5-(1H-pyrrolo[2,3-b]pyridin-3-ylmethyl)-N-[4-(trifluoromethyl)benzyl]pyridin-2-amine 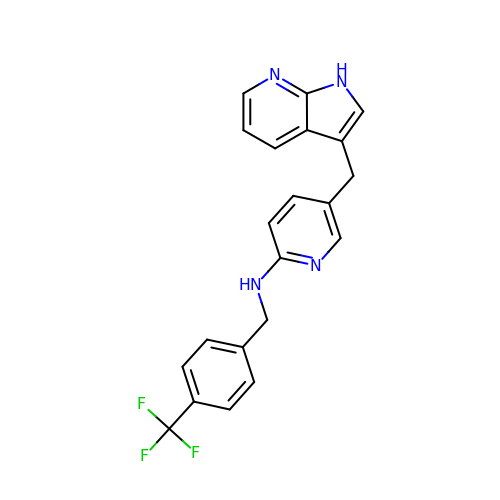| C21 H17 F3 N4 | NODCQQSEMCESEC-UHFFFAOYSA-N> GGVSFSEVMGKQKDEQAREQLKEGMIKIEEQGKKLSETRTQEELQKYVAAVATFALQAGFLGPNLEERRGFNRRGKEEIGKISGEVYLKLLDLKKAVRAKEKKGLDILNMVGEIKGTLER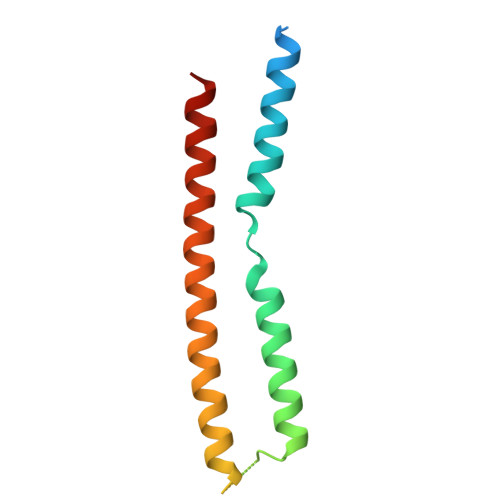VYA> MSVDNAEQIAQAYSWLRAMSGGKLTQEQVTA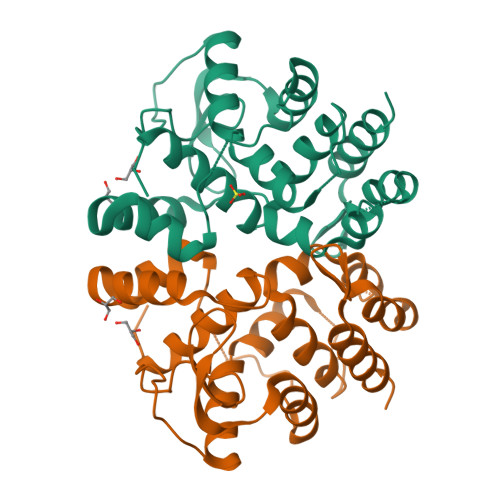GDSIIAMNGLKTFAQVIGYKMSDAVTGFRDISENGYKLIKSFEGFEPKAYQDTGGVWTIGYGTIKYPNGTRVKKGDMCTMAEAEEWLKNDCAWVDACLDKYLKFQPTQNQFDALASFVYNVGETAFSKSTMLKSLNAGNFAGAANQFDKWVYDNGKLIKGLVNRRAAEKKLFLS2-ACETYLAMINO-4-METHYL-PENTANOIC ACID [1-(1-FORMYL-PENTYLCARBAMOYL)-3-METHYL-BUTYL]-AMIDE 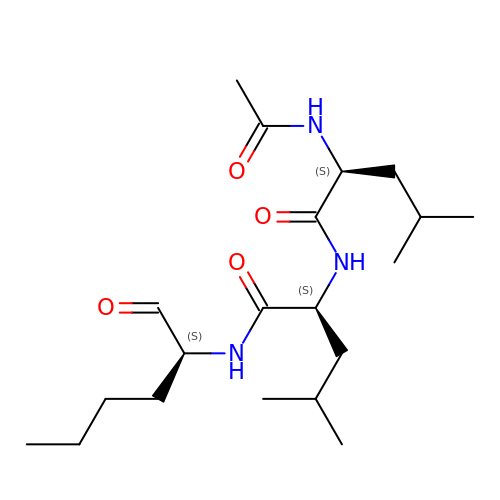| C20 H37 N3 O4 | FMYKJLXRRQTBOR-BZSNNMDCSA-N>PPCDSIVVAYYFCGEPIPYETLVRGRAVTLGQFKELLTKKGSYRYYFKKVSDEFDCGVVFEEVREDEA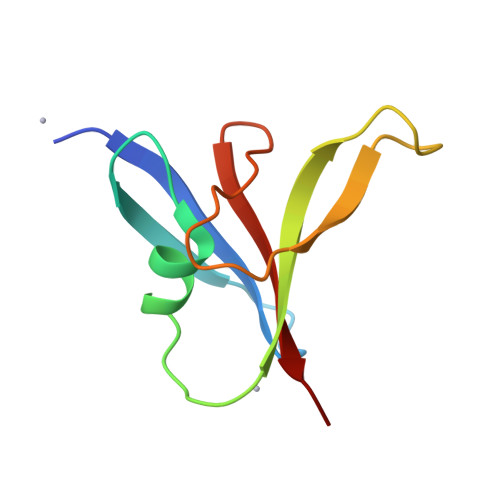ILPVFEEKIIGKVEKVD[6x]Mammalian reovirus (MRV) is the prototypical member of genus Orthoreovirus of family Reoviridae. Here, we report the 3.3 Å-resolution asymmetric reconstruction of transcribing MRV and in situ atomic models of its capsid proteins, the asymmetrically attached RNA-dependent RNA polymerase (RdRp) λ3, and RdRp-bound nucleoside triphosphatase μ2 with a unique RNA-binding domain. All viruses in the Reoviridae are capable of transcribing RNA inside intact capsids (endogenous transcription) without the need of host factors, an attracting characteristic that allows viral RNA transcription of these viruses to be studied in vitro in cell-free environment. The ISVP transcribes its ten genomic segments, adds a methylated guanosine cap to the 5′ end of each mRNA transcript, and releases the capped mRNA from the turrets at the capsid vertices.

Each asymmetric unit is composed of three and one third μ1 trimers—Q, R, S, and 1/3T trimers—totaling ten μ1 monomers. Our asymmetric reconstruction reveals two types among the ten N-myristoyl fragments in each asymmetric unit: nine are at the interface between two μ1 trimers, and one is at the interface between μ1 and λ2. Notably, the N-myristoyl group of the first type is kept within each respective μ1’s hydrophobic pocket, a helix-loop-helix motif (residue M212–R243). In contrast, the N-myristoyl group of the second type is exposed and extended to interact with λ2. The different conformations arise from the different positioning of the interacting loops of Domain I—namely, Loop 51–61 and Loop 72–96, which face toward the virus core. The bond is formed via complementarity between Loop 51–61 of one μ1 trimer and Loop 72–96 of its neighboring μ1 trimer. Five λ2 subunits form a pentameric turret with an axial channel. In our structure of ISVP, loop 581–588 of λ2 bends towards the 5-fold axis (green in Fig. 7d, e) to avoid steric clash with N-myristoyl fragments of μ1, unlike the unbent loop (gray structures in Fig. 7d, e) in the crystal structure of the core, in which μ1 is absent. When TECs of ISVP are in the transcription initiation state, most of the N-myristoyl fragments of membrane penetration protein µ1 remain hidden inside the hydrophobic pockets. This observation suggests that the trigger for RNA transcription is not the attachment of µ1 to the cell membrane, but rather the removal of protection protein σ3 from the capsid surface.

>GNASSIVQTINVTGDGNVFKPSAETSSTAVPSLSLSPGMLN[10x];> MANVWGVRLADSLSSPTIETRTRQYTLHDLCSDLDANPGREPWKPLRNQRTNNIVAVQLFRPLQGLVLDTQLYGFPGAFDDWERFMREKLRVLKYEVLRIYPISNYSNEHVNVFVANALVGAFLSNQAFYDLLPLLIINDTMIGDLLGTGASLSQFFQSHGDVLEVAAGRKYLQMENYSNDDDDPPLFAKDLSDYAKAFYSDTYEVLDRFFWTHDSSAGVLVHYDKPTNGHHYLLGTLTQMVSAPPYIINATDAMLLESCLEQFSANVRARPAQPVTRLDQCYHLRWGAQYVGEDSLTYRLGVLSLLATNGYQLARPIPRQLTNRWLSSFVSQIMSDGVNETPLWPQERYVQIAYDSPSVVDGATQYGYVRKNQLRLGMRISALQSLSDTPSPVQWLPQYTIDQAAMDEGDLMVSRLTQLPLRPDYGNIWVGDALSYYVDYNRSHRVVLSSELPQLPDTYFDGDEQYGRSLFSLARKIGDRSLVKDTAVLKHAYQAIDPNTGKEYLRSGQSVAYFGASAGHSGADQPLVIEPWIQGKISGVPPPSSVRQFGYDVARGAIVDLARPFPSGDYQFVYSDVDQVVDGHDDLSISSGLVESLLSSCMHATAPGGSFVVKINFPTRPVWHYIEQKILPNITSYMLIKPFVTNNVELFFVAFGVHQHSSLTWTSGVYFFLVDHFYRYETLSTISRQLPSFGYVDDGSSVTGIETISIENPGFSNMTQAARIGISGLCANVGNARKSIAIYESHGARVLTITSRRSPASARRKSRLRYLPLIDPRSLEVQARTILPADPVLFENVSGASPHVCLTMMYNFEVSSAVYDGDVVLDLGTGPEAKILELIPATSPVTCVDIRPTAQPSGCWNVRTTFLELDYLSDGWITGVRGDIVTCMLSLGAAAAGKSMTFDAAFQQLIKVLSKSTANVVLVQVNCPTDVVRSIKGYLEIDSTNKRYRFPKFGRDEPYSDMDALEKICRTAWPNCSITWVPLSYDLRWTRLALLESTTLSSASIRIAELMYKYMPIMRIDIHGLPMEKRGNFIVGQNCSLVIPGFNAQDVFNCYFNSALAFSTEDVNAAMIPQVSAQFDATKGEWTLDMVFSDAGIYTMQALVGSNANPVSLGSFVVDSPDVDITDAWPAQLDFTIAGTDVDITVNPYYRLMTFVRIDGQWQIANPDKFQFFSSASGTLVMNVKLDIADKYLLYYIRDVQSRDVGFYIQHPLQLLNTITLPTNEDLFLSAPDMREWAVKESGNTICILNSQGFVLPQDWDVLTDTISWSPSIPTYIVPPGDYTLTPL;>[10x]PGGVPWIAVGDETSVTSPGALRRMTSKDIPETAIINTDNSSGAVPSESALVPYIDEPLVVVTEHAITNFTKAEMALEFNREFLDKMRVLSVSPKYSDLLTYVDCYVGVSARQALNNFQKQVPVITPTRQTMYVDSIQAALKALEKWEIDLRVAQTLLPTNVPIGEVSCPMQSVVKLLDDQLPDDSLIRRYPKEAAVALAKRNGGIQWMDVSEGTVMNEAVNAVAASALAPSASAPPLEEKSKLTEQAMDLVTAAEPEIIASLVPVPAPVFAIPPKPADYNVRTLRIDEATWLRMIPKSMNTPFQIQVTDNTGTNWHLNLRGGTRVVNLDQIAPMRFVLDLGGKSYKETSWDPNGKKVGFIVFQSKIPFELWTAASQIGQATVVNYVQLYAEDSSFTAQSIIATTSLAYNYEPEQLNKTDPEMNYYLLATFIDSAAITPTNMTQPDVWDALLTMSPLSAGEVTVKGAVVSEVVPADLIGSYTPESLNTSLPNDAARCMIDRASKIAEAIKIDDDAGPDEYSPNSVPIQGQLAISQLETGYGVRIFNPKGILSKIASRAMQAFIGDPSTIITQAAPVLSDKNNWIALAQGVKTSLRTKSLSAGVKTAVSKLSSSESIQNWTQGFLDKVSAHFPAPKPDCPTSGDSGESSNRRVKRDSYAGVVKRGYTR> SHMKFTVEREHLLKPLQQVSGPLGGRPTLPILGNLLLQVADGTLSLTGTDLEMEMVARVALVQPHEPGATTVPARKFFDICRGLPEGAEIAVQLEGERMLVRSGRSRFSLSTLPAADFPNLDDWQSEVEFTLPQATMKRLIEATQFSMAHQDVRYYLNGMLFETEGEELRTVATDGHRLAVCSMPIGQSLPSHSVIVPRKGVIELMRMLDGGDNPLR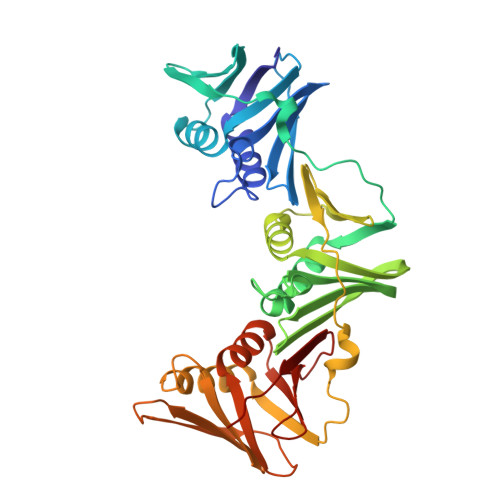VQIGSNNIRAHVGDFIFTSKLVDGRFPDYRRVLPKNPDKHLEAGCDLLKQAFARAAILSNEKFRGVRLYVSENQLKITANNPEQEEAEEILDVTYSGAEMEIGFNVSYVLDVLNALKCENVRMMLTDSVSSVQIEDAASQSAAYVVMPMRL> QIYTDIEM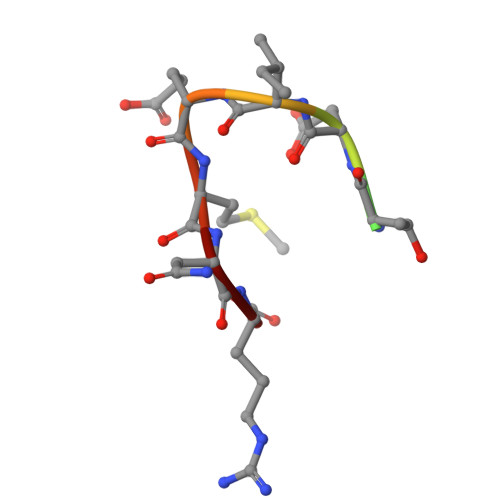NR> GAMGQHHGVTKCNITCSKMTSKIPVALLIHYQQNQASCGKRAIILETRQHRLFCADPKEQWVKDAMQHLD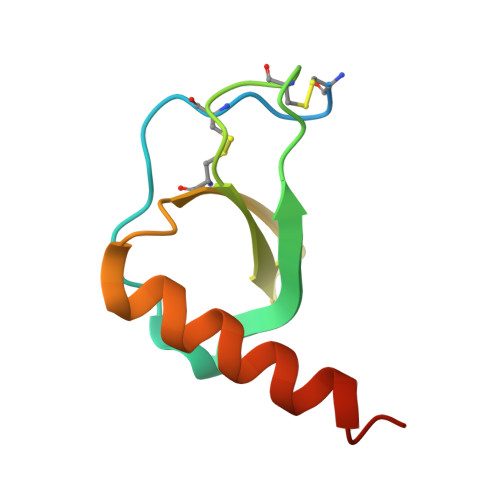RQAAALTRNG>[3x]MPSGSVLVTGGTGY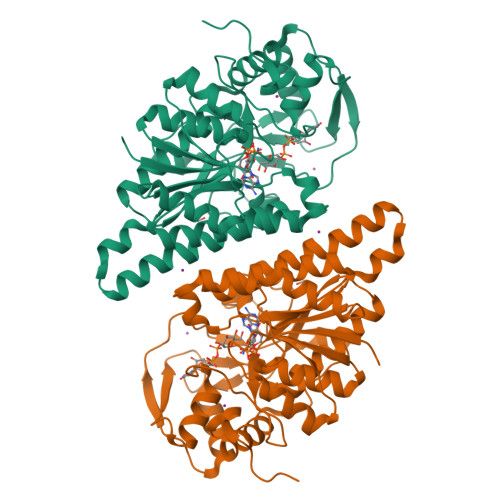IGSFTTLALLEAGYKVVVADNLYNSSAEALNRIELISGKKAEFAQLDVTDEAAFDKVFEAHPDIDSVIHFAALKAVGESGEKPLDYYHVNVYGTICLLRSMVRHNVTNIVFSSSATVYGDATRFPDMIPIPEHCPLGPTNPYGNTKFAIELAITDVINAQRNNAKKAGNETEAAKWNGALLRYFNPAGAHPSGIMGEDPQGVPYNLLPLLAQVATGKREKLLVFGDDYASHDGTAIRDYIHILDLADGHLKALNYLRANNPGVRAWNLGTGRGSTVYEMIRAFSKAVGRDLPYEVAPRRAGDVLNLTSNPTRANTELGWKAQRTLEQACEDLWLWTKNNPQGYRQQPPAELLEQLKK>MQKYVCNVCGYEYDPAEHDNVPFDQLPDDWCCPVC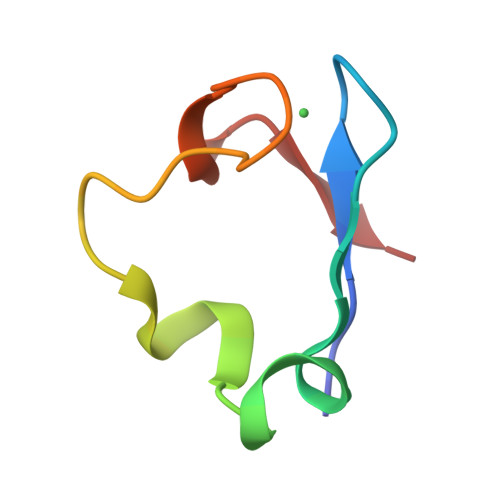GNSKDQFSPA[2x]> GHMGQKASQQLALKDSKEVPVVCEVVSEAIVHAAQKLKEYLGFEYPPSKLCPAANTLNEIFLIHFITFCQEKGVDEWLTTTKMTKHQAFLFGADWIWTFWGSDKQIKLQLAVQTLQMSSPPPVESKPCDLSNPESRVEESSWKKSRFDKLEEFCNLIGEDCLGLFIIFGMPGKPKDIRGVVLDSVKSQMVRSHLPGGKAVAQFVLETEDCVFIKELLRNCLSKKDGLREVGKVYISIL;> MAHHHHHHSSGASAQDARYGQKDSSDQNFDYMFKLLIIGNSSVGKTSFLFRYADDSFTSAFVSTVGIDFKVKTVFKNEKRIKLQIWDTAGQERYRTITTAYYRGAMGFILMYDITNEESFNAVQDWSTQIKTYSWDNAQVILVGNKCDMEDERVISTERGQHLGEQLGFEFFETSAKDNINVKQTFERLVDIICDKMSESLETDPAITAAKQNTRLKETPPPPHPNCGC

One such Rab15 effector is Rep15, which is known to have a role in receptor recycling from the endocytic recycling compartment but otherwise remains poorly characterized. Biochemical validation of the interactions is presented and crystal structures of the Rep15:Rab3B and Rep15:Rab3C complexes provide additional mechanistic insight. We find that Rep15 adopts a globular structure that is distinct from other reported Rab15, Rab3 and Rab34 effectors. Detailed biochemical studies reveal that Rep15 is selective for Rab15, Rab3 paralogs and Rab34 and does not bind to other evolutionarily similar Rab GTPases.

The structure is composed of one Rep15:Rab3CGppNHp_Q222H_10-227 complex per asymmetric unit. The structure of Rep15:Rab3C reveals that, unlike most Rab effectors, Rep15 is a single domain globular protein which presumably explains why the other three deletion Rep15 constructs were not soluble. No electron density was observed for the first 14 amino acids, the middle 117 to 130 amino acids and for the last residue. No electron density was observed for the first 16 amino acids and the last 30 amino acids of Rab3CGppNHP_Q222H_10-227 (bovine). Rep15 is composed of 7α-helices and 7β-strands. The central core is made by the β-strands which are flanked by the α-helices. Similar to all known Rab:effector complexes, switch I, switch II and the interswitch regions of Rab3C are at the interface with the effector. They interact with the α3 and α4 helices of Rep15, constituting the primary binding site, with a second site being composed of a loop (residues 115 to 145), ß2 and β3 of Rep15. α3 of Rep15 interacts with the switch I and interswitch regions, while α4 and β3 interact with the switch II region of Rab3C. Analysis of the interface by PDBePISA40 revealed that the Rep15:Rab3C complex has a total buried interface of 843.4 Å2. The hydrophobic patch is composed of switch I (V63 and I65), interswitch residues (F67 and W84) and switch II residues (Y92, I95 and Y99) that interact with the hydrophobic side chains of L88Rep15, F89Rep15 from α3 and F151Rep15, L154Rep15 and I155Rep15 from α4.> STDNAETGVIEAGNTDTDFSGELAAPGSNHTNVKFLFDRSRLLNVIKVLEKDAVFPRPFPTATGTQQDDGYFCLLTPRPTVASRPATRFGLYVSPSDSGVLANTSLDFNFYSLACFTYFRSDLEVTVVSLEPDLEFAVGWFPSGSEYQASSFVYDQLHVPYHFTGRTPRAFASKGGKVSFVLPWNSVSSVLPVRWGGASKLSSATRGLPAHADWGTIYAFIP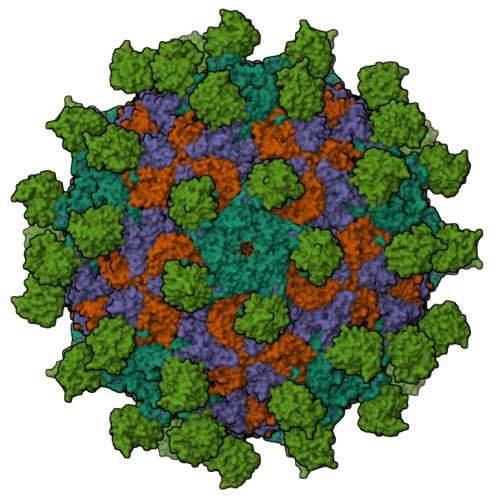RPNEKKSTAVKHVAVYIRYKNARAWCPSMLPFRSYK;> DRVTTQTAGNTAINTQSSLGVLCAYVEDPTKSDPPSSSTDQPTTTFTAIDRWYTGRLNSWTKAVKTFSFQAVPLPGAFLSRQGGLNGGAFTATLHRHFLMKCGWQVQVQCNLTQFHQGALLVAMVPETTLDVKPDGKAKSLQELNEEQWVEMSDDYRTGKNMPFQSLGTYYRPPNWTWGPNFINPYQVTVFPHQILNARTSTSVDINVPYIGETPTQSSETQNSWTLLVMVLVPLDYKEGATTDPEITFSVRPTSPYFNGLRNRYTT;> GPIPTAPRENSLMFLSTTPDDTVPAYGNVRTPPVNYLPGEITDLLQLARIPTLMAFGRVPEPEPASDAYVPYVAVPTQFDDKPLISFPITLSDPVYQNTLVGAISSNFANYRGCIQITLTFCGPMMARGKFLLSYSPPNGTQPQTLSEAMQCTYSIWDIGLNSSWTFVIPYISPSDYRETRAITNSVYSADGWFSLHKLTKITLPPDCPQSPCILFFASAGEDYTLRLPVDCNPSYVFH;> GNVQTTSKNDFDSRGNNGNMTFNYYANTYQNSVDFSTSSSASGAGPGNSRGGLAGLLTNFSGILNPLGYLK;> SMACYGGFDLYFILDKSGSVLHHWNEIYYFVEQLAHKFISPQLRMSFIVFSTRGTTLMKLTEDREQIRQGLEELQKVLPGGDTYMHEGFERASEQIYYENRQGYRTASVIIALTDGELHEDLFFYSEREANRSRDLGAIVYAVGVKDFNETQLARIADSKDHVFPVNDGFQALQGIIHSILKKSC> MSDVAIVKEGWLHKRGEYIKTWRPRYFLLKNDGTFIGYKERPQDVDQREAPLNNFSVAQCQLMKTERPRPNTFIIRCLQWTTVIERTFHVETPEEREEWT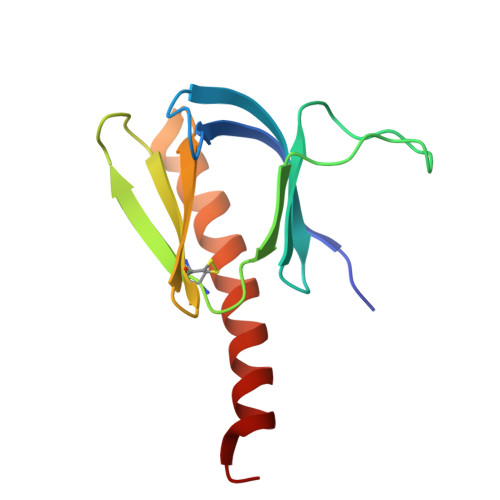TAIQTVADGLKKQEEEEMDFR>MPSDVASSTGLPTPWTVRYSKSKKREYFFNPETKHSQWEEPEGTNKDQLHKHLRDHPVRVRCLHILIKHKDSRRPASHRSENITISKQDATDELKTLITRLDDDSKTNSFEALAKERSDCSSYKRGGDLGWFG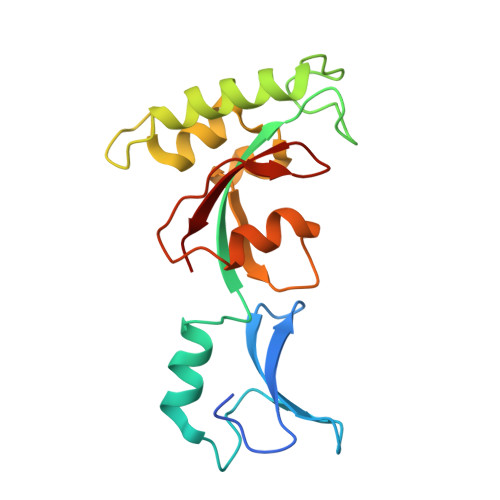RGEMQPSFEDAAFQLKVGEVSDIVESGSGVHVIKRVG[2x]> GPDSMEVEESLLDALLGKALAGDQMNSRIEGLFE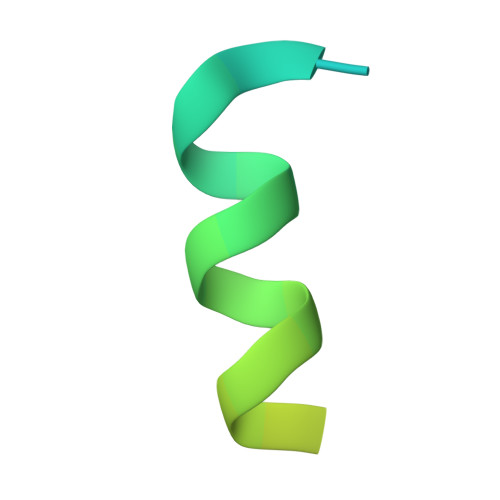DLD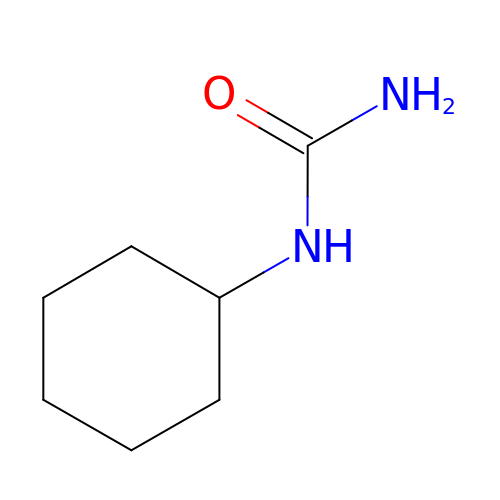N-cyclohexylurea | C7 H14 N2 O | WUESWDIHTKHGQA-UHFFFAOYSA-N>DERDRVQKKTFTKWVNKHLIKAQRHISDLYEDLRDGHNLISLLEVLSGDSLPREKGRMRFHKLQNVQIALDYLRHRQVKLVNIRNDDIADGNPKLTLGLIWTIILHFQISDIQVSGQSEDMTAKEKLLLWSQRMVEGYQGLRCDNF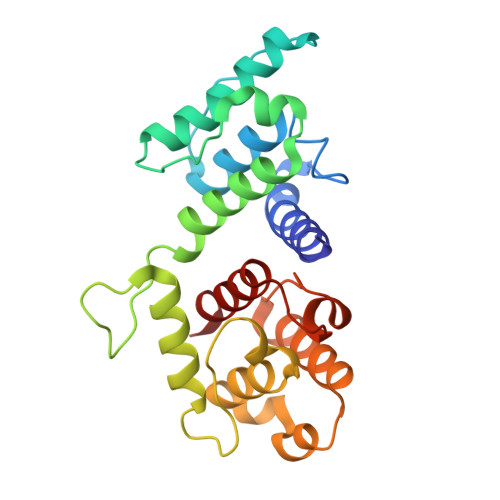TSSWRDGRLFNAIIHRHKPLLIDMNKVYRQTNLENLDQAFSVAERDLGVTRLLDPEDVDVPQPDEKSIITYVSSLYDAMP[2x]>MSESPMFAANGMPKVNQGAEEDVRILGYDPLASPALLQVQIPATPTSLETAKRGRREAIDIITGKDDRVLVIVGPCSIHDLEAAQEYALRLKKLSDELKGDLSIIMRAYLEKPRTTVGWKGLINDPDVNNTFNINKGLQSARQLFVNLTNIGLPIGSEMLDTISPQYLADLVSFGAIGARTTESQLHRELASGLSFPVGFKNGTDGTLNVAVDACQAAAHSHHFMGVTKHGVAAITTTKGNEHCFVI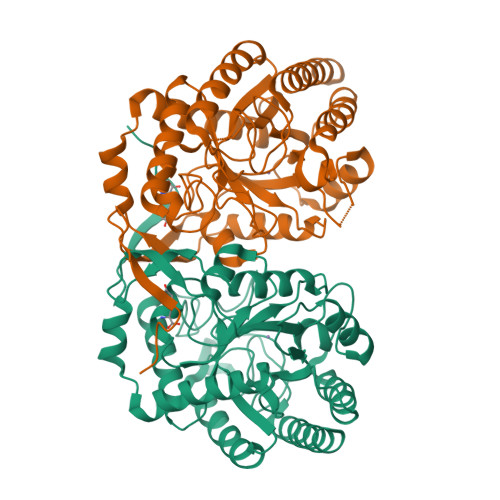LRGGKKGTNYDAKSVAEAKAQLPAGSNGLMIDYSHGNSNKDFRNQPKVNDVVCEQIANGENAITGVMIESNINEGNQGIPAEGKAGLKYGVSITDACIGWETTEDVLRKLAAAVRQRREVNKK[8x]>[9x]MSAKAAEGYEQIEVDVVAVWKEGYVYENRGSTSVDQKITITKGMKNVNSETRTVTATHSIGSTISTGDAFEIGSVEVSYSHSHEESQVSMTETEVYESKVIEHTITIPPTSKFTRWQLNADVGGADIEYMYLIDEVTPIGGTQSIPQVITSRAKIIVGRQIILGKTEIRIKHAERKEYMTVVSRKSWPAATLGHSKLFKFVLYEDWGGFRIKTLNTMYSGYEYAYSSDQGGIYFDQGTDNPKQRWAI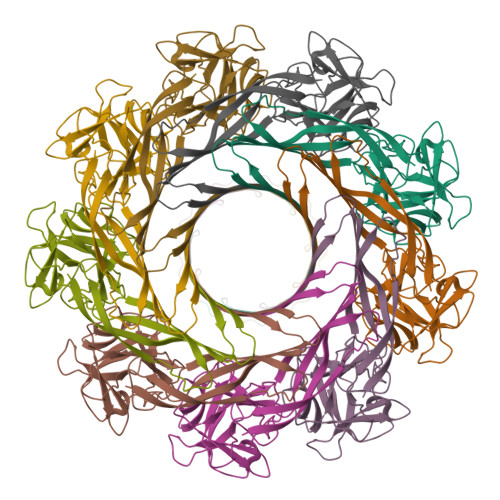NKSLPLRHGDVVTFMNKYFTRSGLCYDDGPATNVYCLDKREDKWILEVVGLVPRGSGHHHHHH> GPHMEDENILRNAVNLQVLKFHYPEIESIIDIASHVAVYQFDVGSQKWLKTSIEGTFFLVKDQRARVGY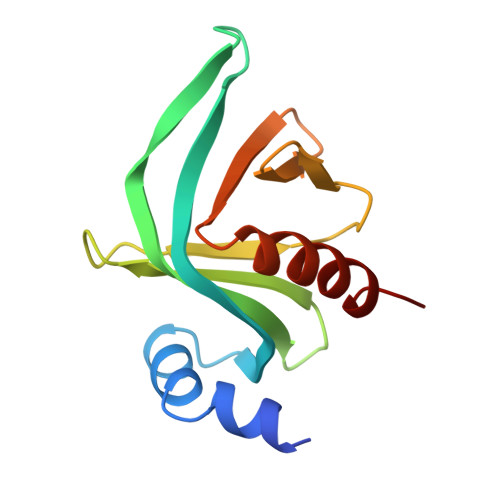VILNRNSPENLYLFINHPSNVHLVDRYLIHRTENQHVVGLWMFDPNDMSRIFNIVKESLLR> MIKLMVGSFAEKKLKRGVQLLSSRDYPNLNLDNQVVQLYSDADIFLGTAYLSKQNKGVGWLISPKKVSLNVTYFIKLFQWSKDKRKNFAHSKLTTAYRLFNQDGDSFGGVTIDCYGDFVLFSWYNSFVYQIRDEIVAAFRQVYPNFLGAYEKIR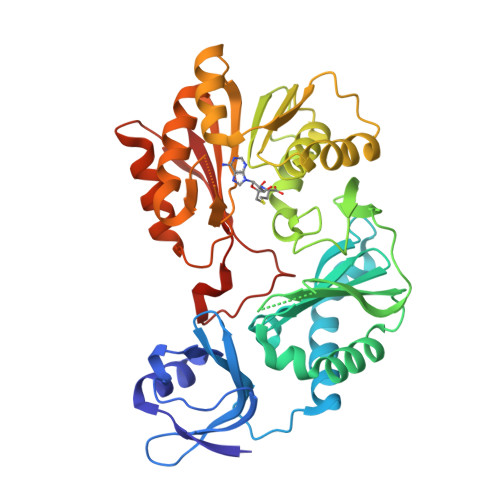FKGIDNVSAHLYGQEAPEQFLILENGISYNVFLNDGLMTGIFLDQRQVRNELINGSAAGKTVLNLFSYTAAFSVAAAMGGAMATTSVDLAKRSRALSLAHFEANHLDMANHQLVVMDVFDYFKYARRHHLTYDIIIIDPPSFARNKKEVFSVSKDYHKLIRQGLEILSENGLIIASTNAANMTVSQFKKQIEKGFGKQKHTYLDLQQLPSDFAVNVQDESSNYLKVFTIKV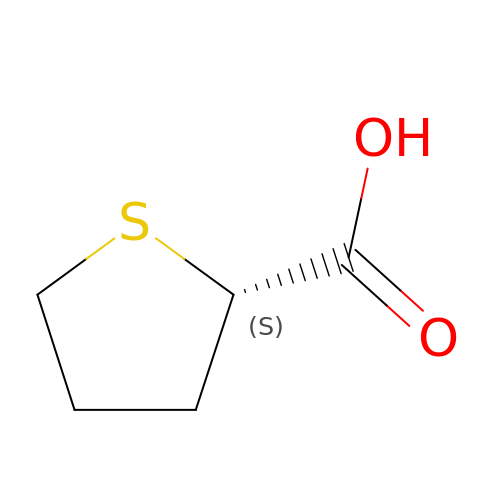(2S)-thiolane-2-carboxylic acid | C5 H8 O2 S | MZOYMQRKTJRHGJ-BYPYZUCNSA-N5-amino-1-~{tert}-butyl-3-(3-methoxyphenyl)pyrazole-4-carboxamide 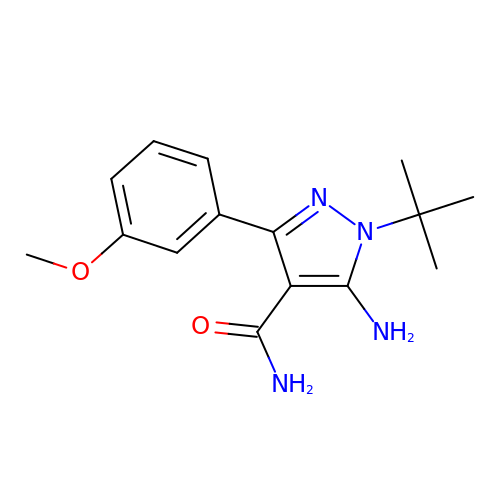| C15 H20 N4 O2 | QDGDUSBCURLURJ-UHFFFAOYSA-N> NHLFAPEAPVSLTIHGSDQTFPVRRVYCVGRNYAAHAREMGFDPEREPPFFFCKPADAVVPVAAGSTLELAYPSQTGNYHYEIELVAAIGKGGCDIPLEQAEEHVWGYAVGLDMTRRDLQMRMREMGR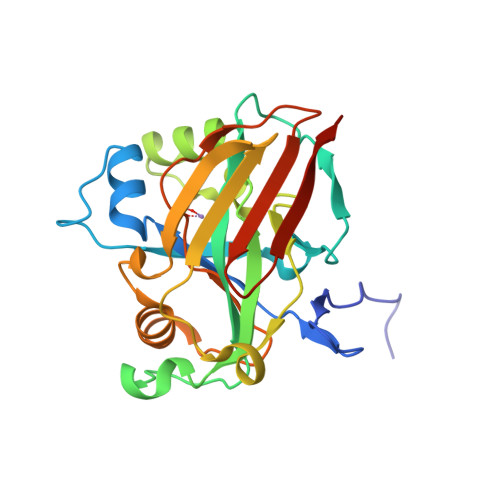PWEIGKAFDRSAPIGPLYPASQVGHPRHAAISLQVDGEDRQRSDIDQLIWSVAETVSYLSRFFELRPGDLVFTGTPEGVGAVERGERMLGAIDGLGELSVRVVLEHHHHHH O-[2-(1,3-dioxo-1,3-dihydro-2H-isoindol-2-yl)ethyl] (4-chlorophenyl)thiocarbamate | C17 H13 Cl N2 O3 S | 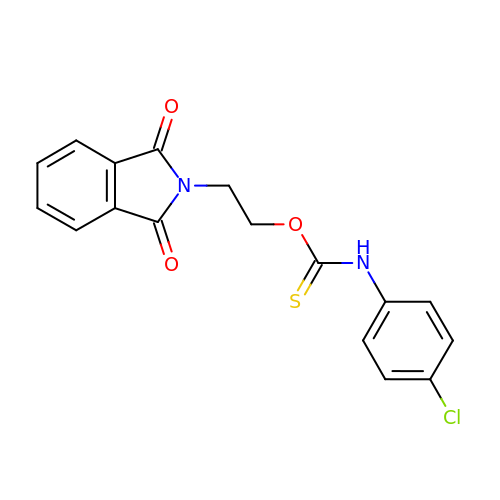BWRRXOIACQYNEK-UHFFFAOYSA-N> SEKEKVEELAQRIREQLPDTELAREAQELADEARKSDDSEALKVVYLALRIVQQLPDTELAREALELAKEAVKSTDSEALKVVELALKIVQQLPDTELAKEALKLAKEAVKSTDSEALKVVELALEIVQQLPDTELAKEALELAEEAVKSTDSEALKVVKLALEIVQQLPDTELA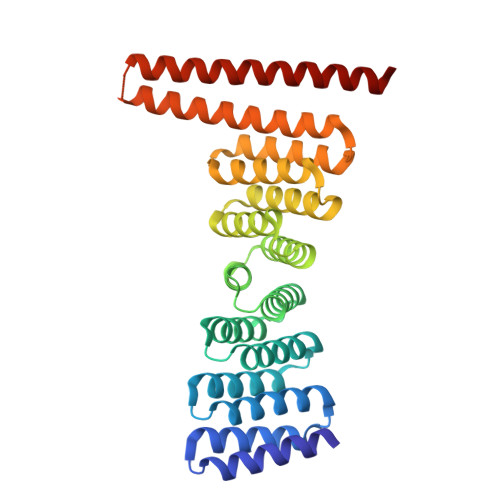REALELAKEAVKSTDSEALKVVYLALRIVQQLPDTELARLALELAKKAVEMTAQEVLEIARAALKAAQAFPNTELAELMLRLAEVAARVMKELERNDEEIKKSDELDDESLLEDIVELLKEIIKLWKILVEVSDVMLKLIS>[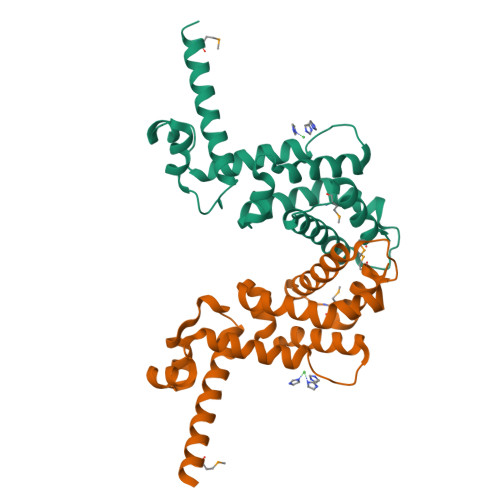4x]SNAMVKDRQIQKTKVAIYNAFISLLQENDYSKITVQDVIGLANVGRSTFYSHYESKEVLLKELCEDLFHHLFKQGRDVTFEEYLVHILKHFEQNQDSIATLLLSDDPYFLLRFRSELEHDVYPRLREEYITKVDIPEDFLKQFLLSSFIETLKWWLHQRQKMTVEDLLKYYLTMVER> MLNPIVRKFQYGQHTVTLETGMM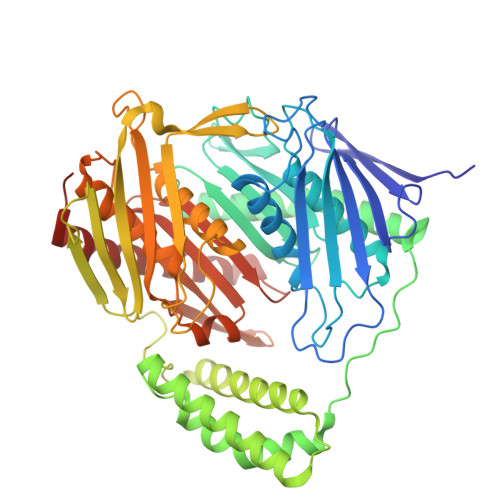ARQATAAVMVSMDDTAVFVTVVGQKKAKPGQDFFPLTVNYQERTYAAGRIPGSFFRREGRPSEGETLIARLIDRPIRPLFPEGFVNEVQVIATVVSVNPQVNPDIVAMIGASAALSLSGIPFNGPIGAARVGYINDQYVLNPTQDELKESKLDLVVAGTEAAVLMVESEAQLLSEDQMLGAVVFGHEQQQVVIQNINELVKEAGKPRWDWQPEPVNEALNARVAALAEARLSDAYRITDKQERYAQVDVIKSETIATLLAEDETLDENELGEILHAIEKNVVRSRVLAGEPRIDGREKDMIRGLDVRTGVLPRTHGSALFTRGETQALVTATLGTARDAQVLDELMGERTDTFLFHYNFPPYSVGETGMVGSPKRREIGHGRLAKRGVLAVMPDMDKFPYTVRVVSEITESNGSSSMASVCGASLALMDAGVPIKAAVAGIAMGLVKEGDNYVVLSDILGDEDHLGDMDFKVAGSRDGISALQMDIKIEGITKEIMQVALNQAKGARLHILGVMEQAINAPRGDIS> STNDNIKDLLDWYSSGSDTF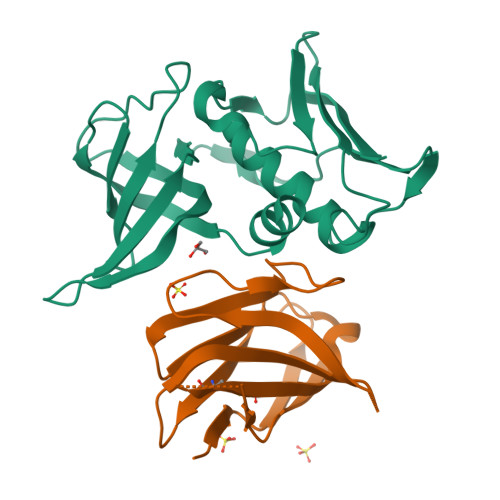TNSEVLDNSLGSMRIKNTDGSISLIIFPSPYYSPAFTKGEKVDLNTKRTKKSQHTSEGTYIHFQISGVTNTEKLPTPIELPLKVKVHGKDSPLKYWPKFDKKQLAISTLDFEIRHQLTQIHGLYRSSDKTGGYWKITMNDGSTYQSDLSKKFEYNTEKPPINIDEIKTIEAEIN;> GAVVSQHPSRVIVKSGTSVKIECRSLDFQATTMFWYRQFPKQSLMLMATSNEGSKATYEQGVEKDKFLINHASLTLSTLTVTSAHPEDSGFYICSALAGSGSSTDTQYFGPGTRLTVL> MLFSNKVIELMHSGDGGSGAEIKMPIDFYQLPGSPPCRAVALTAAALDIEMNFKQVNLMNGEHLKPEFLKINPQHTIPTIDDNGFRLWESRAIMTYLADQYGKNDTLYPKDLKKRAIVNQRLYFDMCSLYKSFMDYYYPIIFMKAVKDQAKYENIGTALSFLDKFLEGENYVAGKNMTLADLSIVSTVSTLEALDYDLSKYKNVTRWFAKIKPEIP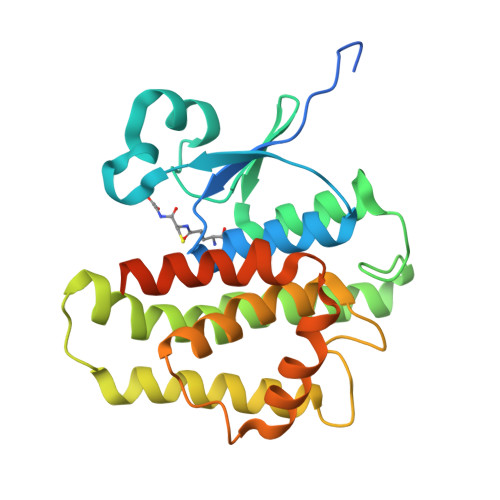KYEEYNNAGLKMFKELVNEKLSKKNLYFQSGSHHHHHH> METRQMAVEQTTGAVTNQTETSWHSIDWAKANREVKRLQVRIAKAVKEGRWGKVKALQWLLTHSFYGKALAVKRVTDNSGSKTPGVDGITWSTQEQKAQAIKSLRRRGYKPQPLRRVYIPKASGKQRPLGIPTTKDRAMQALYALALEPVAETTADRNSYGFRQGRCTADAAGQCFTVLGRSDCAKYILDADITGCFDNISHEWLLDNIPLDKEVLRKWLKSGFVWKQQLFPTHAGTPQGGVISPMLANMTLDGMEELLKKHLRKQKVNLIRYADDFVVTGESK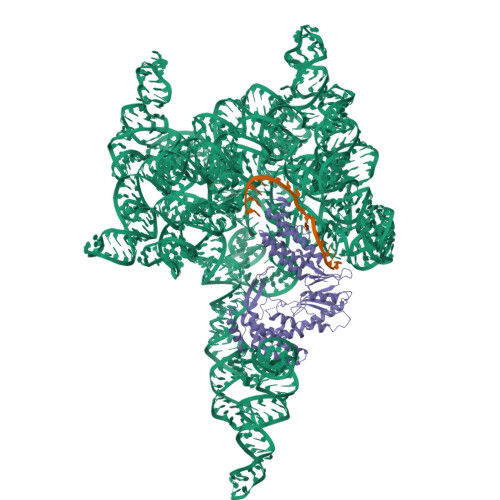ETLEKVTTVIQEFLKERGLTLSEEKTKVVHIEEGFDFLGWNIRKYGEKLLIKPAKKNIKAFHKKIRDALKELRTATQEAVIDTLNPIIKGWANYHRNQVSKRIFNRADDNIWHKLWRWAKRRHPNKPARWTKNKYFIKIGNRHWVFGTWKKDKEGRLRSRYLIKAGDTRIQRHVKIKADANPFLPEWAEYFEERKKLKEAPAQYRRIRRELWKKQGGICPVCGGEIEQDMLTEIHHILPKHKGGSDDLDNLVLIHANCHKQVHSRDGQHSRFLLKEGL>[4x]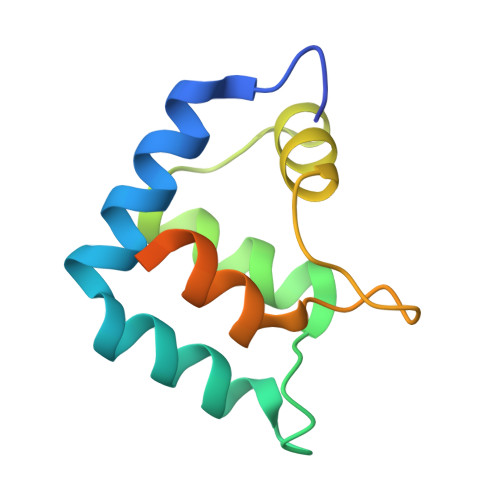GPHMATADRDILARLHKAVTSHYHAITQEFENFDTMKTNTISREEFRAICNRRVQILTDEQFDRLWNEMPVNAKGRLKYPDFLSRFSSETAATPMATGDSAVAQR> GSHMSSLPVPYKLPVSLSVGSCVIIKGTPIHSFINDPQLQVDFYTDMDEDSDIAFRFRVHFGNHVVMNRREFGIWMLEETTDYVPFEDGKQFELCIYVHYNEYEIKVNGIRIYGFVHRIPPSFVKMVQVSRDISLTSVCVCN

Galectin-13 (Gal-13, a.k.a. placental protein 13 or PP13) was first isolated from human placenta, and its gene has been mapped to chromosome 19q13.1, which is in close proximity to the galectin-4, -7, -10 and 1412 genes. As with all other galectins, Gal-13 adopts the typical “jelly-roll” fold formed by sandwiching two anti-parallel β-sheets that consist of six (S1-S6) and five (F1-F5) β-strands and a short α-helix connecting strands S2 and F5. Gal-13 crystallizes as a dimer with its subunit interface formed by the last five C-terminal residues (Val135, Cys136, Val137, Cys138, and Asn139) that are located within the F1 β-strand. We found that Gal-13 forms a homodimer structure that is stabilized primarily by the presence of two disulfide bonds, unlike the structures of other prototype galectins.

We crystallized wild-type Gal-13 and its R53H mutant using two different conditions. The wild-type lectin was crystallized in a solution containing PEG 4000. Our Gal-13 structure shows that Arg53 protrudes from the base of the carbohydrate binding site, and the characteristics of an arginine, including its size and charge, are obviously different from those of a histidine. This difference suggests that wild type Gal-13 should not be able to bind galactose, which likely explains why we could not find lactose bound to Gal-13 in crystals exposed even to 50 mM lactose. Even with 50 mM lactose in the crystallization buffer, our Gal-13 structure lacks any electron density that is expected for a bound lactose molecule and only shows water molecules in the ligand binding site. However, our research shows that galactose, maltose, xylose, arabinose, glucose, mannose, lactose, fructose, sucrose, and cellulose do not inhibit Gal-13-mediated agglutination. Moreover, our biochemical results indicate that Gal-13 may not bind carbohydrates, a proposal that is consistent with previous work demonstrating that Gal-13 purified from human term placenta contains no carbohydrate at all.>MRGSHHHHHHGSLVPRGSMKKVSVIMPTFNNGEKLHRTISSVLNQTMKSTDYELIIIDDHSNDNGETLNVIKKYKGLVRFKQLKKNSGNASVPRNTGLKMSKAEYVFFLDSDDLLHERALEDLYNYGKENNSDLIIGKYGVEGKGRSVPKAIFEKGNVAKADIIDNSIFYALSVLKMFKKSVIDKNKIKFKTFSKTAEDQLFTIEFLMNSKNYSIKTDYEYYIVVNDFESSNHLSVNKSTGNQYFATINEIYKAIYKSPIYKNQEKRHQLAGKYTTRLLRHGQKKNFANSKMKYEDKIEWLNNFSKTINKV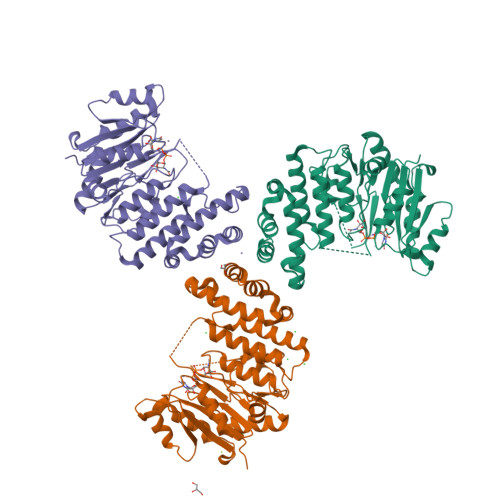PRDSDKYVTQIFNLKLEAIRQNDLLAVMIADKLL[3x]> VNFEEVRELVPQKYPFLFIDKVIELQKESRIVCLKNISGNEPFFA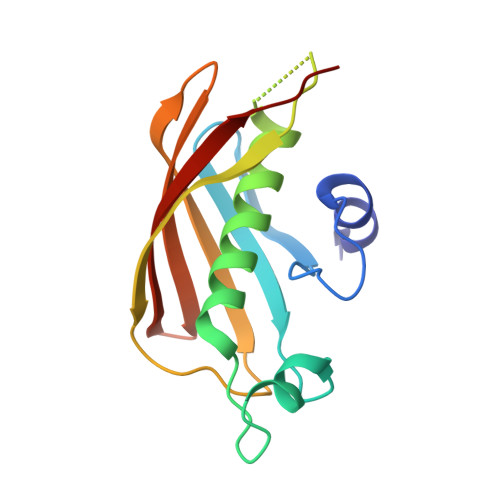GHFPDFAIMPGVLIVEALAQASIILFKKSFSTEQHKDKVFLLASANVRFSKPVFPGDQLILEIDIEKVISSAAIVKGVAKVGDKVVTKATLSFGVANKD>MAKKTSSQPGSRPPGPFPWPLIGNAAEVGSAPHLSFARLARRYGDVFQIRLGSCPVVVLNGERAIRQALVQQGAAFAGRPPFPSFQVVSGGRSLAFGRYSERWKVQRRVAHSTVRAFSTGQPRSRRVLEQHVLGEARELVRLLVRGSAGGAFLDPAPLTVVAVANVMSAVCFGCRYSHDDAEFRGLLSHNEKFGRTVGAGSLVDVLPWLQRFPNPVRTAFRDFQQLNRDFYSFVLDKFLRHRSSLRPGAAPRDMMDAFIHTVGKEEAEGNGDSGPRLDLEYVPATVTDIFGASQDTLSTALQWLLILFTRYPEVQARVQEELDRVVGRDRLPCMDDQPHLPYVMAFLYEAMRFSSFVPVTIPHATTADTSIMGYHIPKDTVVFVNQWSVNHDPVKWPNPEDFNPARFLDKNGFINKDLA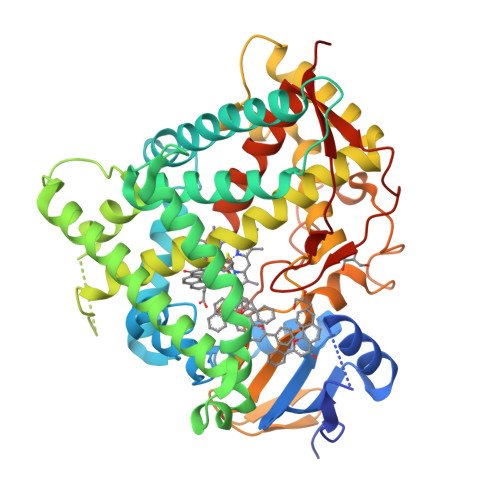SSVMIFSVGKRRCIGEELSKMQLFLFISILAHQCNFRANPDEDSKMDFSYGLTIKPKSFTINVTLRSTHHHHHH[2x]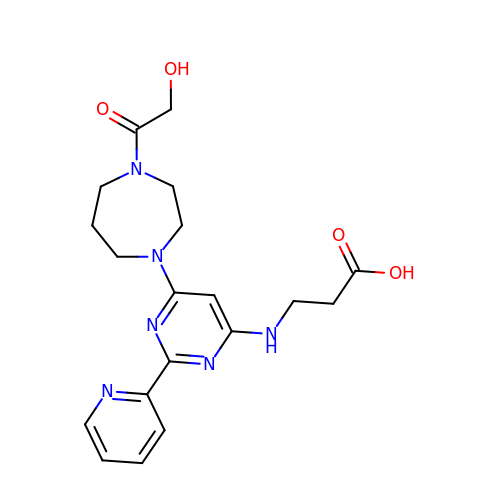N-{6-[4-(hydroxyacetyl)-1,4-diazepan-1-yl]-2-(pyridin-2-yl)pyrimidin-4-yl}-beta-alanine | C19 H24 N6 O4 | BFXYLSMGFITUJF-UHFFFAOYSA-N3,3-DICHLORO-2-PHOSPHONOMETHYL-ACRYLIC ACID | C4 H5 Cl2 O5 P | 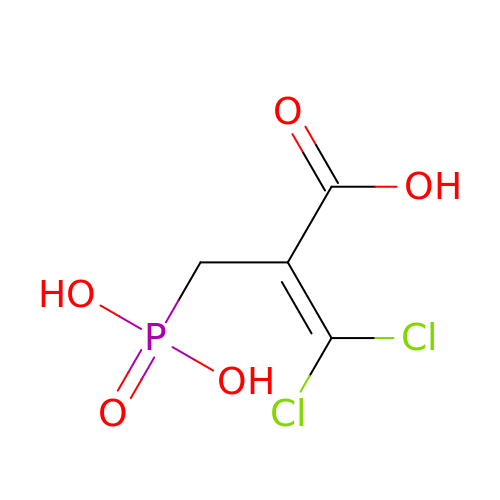IBGSKYLUHGAGLB-UHFFFAOYSA-N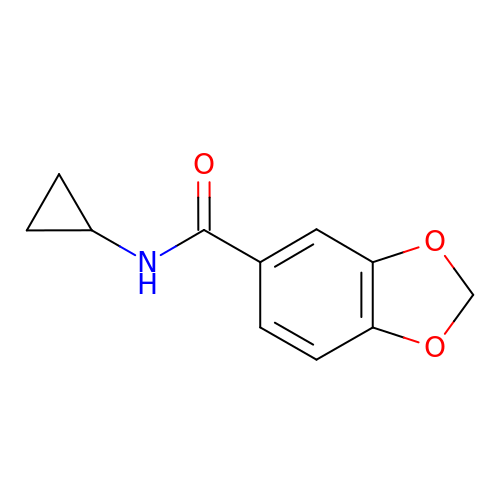~{N}-cyclopropyl-1,3-benzodioxole-5-carboxamide | C11 H11 N O3 | OUGQMSXIPFSZBI-UHFFFAOYSA-N Enzymes of the vanillyl alcohol oxidase/p-cresol methyl hydroxylase (VAO/PCMH) superfamily are found across all kingdoms where they perform a range of metabolic functions. These flavoproteins share a conserved FAD-binding domain and a more variable substrate-binding domain that enables interactions with a range of substrates. One of these, the 4-phenol oxidases/dehydrogenases, catalyzes the oxidation of para-substituted phenolic compounds. A fundamental distinction is that the oxidases efficiently react with oxygen producing hydrogen peroxide whereas the dehydrogenases hardly react with oxygen and typically employ other proteins, such as cytochrome c, as acceptors.

We further studied the P151G mutation to assess the effect of removing en bloc the side chain, and P151N and P151T to test the introduction of hydrogen-bonding groups. The P151G mutation was found to elicit the same oxidase-activating effect of P151L whereas P151T and P151N conserve the properties of a dehydrogenase. Spectrophotometric measurements confirmed that the vanillyl alcohol-reduced P151N and P151T proteins are hardly re-oxidized by molecular oxygen though they retain dehydrogenase activity while P151G can effectively turn over using oxygen as co-substrate and the product is formed. In general, the oxidase-active variants (P151L, P151G, P151I, P151V) all adopt the trans conformation that slightly shifts the amino acid at position 151 away from the flavin. The analysis revealed a consistent pattern: in the oxidase mutants, the 150-153 loop conformations create tunnels that lead to the flavin re side.

>[3x]MAAPLPEGVSAEAMSSALDRFARIVGADWVFTEDKITPYEDPYTISNDETEHRPYAAVAPASTEEVQEIVRVANEFGVPLWPVSRGKNFAYGGAAPVMSGTVVLDMNRMNRILEVNEEFGYALVEPGVSYFELYDYIQEKGLKLWIDVPDGGWGSVVGNALDHGIGYTPYGDHFAMQCGMEVVLPNGEVVRTGMGAMPGNNTWQLFKYGYGPYVDGIFSQSNFGVVTKMGIWLMPEPAGYRPYLITFENEDDIETVTERLRPLKVAGVIQNGATVRSLVLDAAITRTKSQYYDGDGPIPPSVAKTMMADLDLGMWNFCGALYGPPPVMDTLWTAIRDSFADIPGVKFYFPEDRRHKVDLLLHRAETMKGVPKLTEFNFLNWDGGGGHVGFSPVSPITGKDAIKQYNMVSSRVREYGFDYMGLLAIGWRDLHHVTVIVYDKTDPDERKKLDELFNILVDEAAAEGYGEYRTHIRYMDRIAKTYSWNDNALWKMHETIKDALDPNGILAPGKSGIWGKNRRKA> AAAAAAAAAAAAAAAAAAAAAAAAAAAAAAAAAAAAAAAAAAAAAAAAAAAAAAAAAAAAAAAAAAAAAAAAAAAAAAAAAAAAAAAAAAAAAAAAAAAAAAAAAAAAAAAAAAAAAAAAAAAAAAAAAAAAAAAAAAAAAAAAAAAAAAAAAAAAAAAAAAAAAAAAAAAAAAAAAAAAAAAAAAAAAAAAAAAAAAAAAAAAAAAAAAAAAAAAAAAAAAAAAAAAAAAAAAAAAAAAAAAAAAAAAAAAAAAAAAAAAAAAAAAAAAAAAAAAAAAAAAAAAAAAAAAAAAAAAAAAAAAAAAAAAAAAAAAAAAAAAAAAAAAAAAMRNLMRCLIMIKSLIKGVDMSRKLAKTRILGYGLMICFLA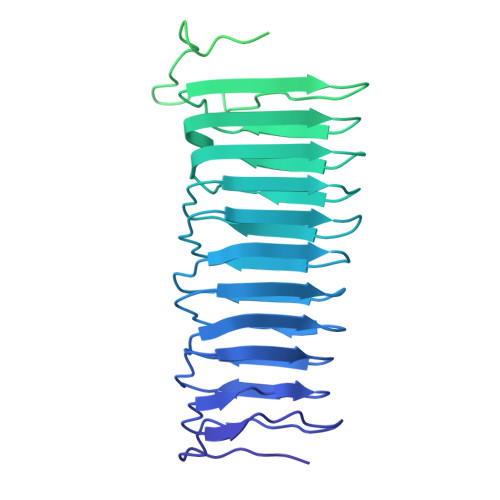GCFHPPYNNFQPDRRAVKRVGVDTGIGAVAGAIASGTASGTLIGAAAGGTVGLVASIYRDSKRKIIRDLQKQDIQYVEYGDTRTLIIPTDKYFMFSSPRLNEICYPGLNNVIRLLNFYPQSTIYVAGFTDNVGSRSHKRKLSQAQAETMMTFLWANGIAAKRLKAEGYGDKNAISDNAIIHGSAQNRRIEIQWFTSPAQPPQPQMAYVK> IVGGQECKDGECPWQALLINEENEGFCGGTILSEFYILTAAHCLYQAKRFKVRVGDRN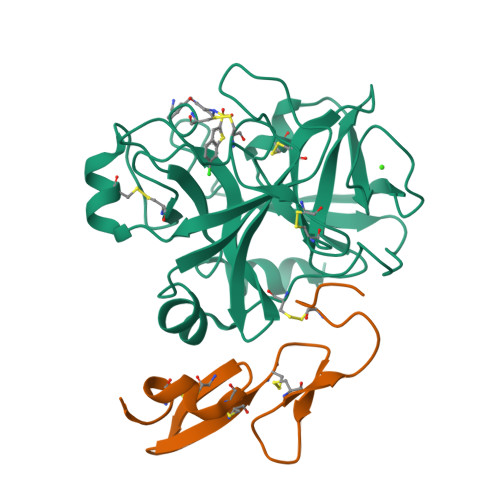TEQEEGGEAVHEVEVVIKHNRFTKETYDFDIAVLRLKTPITFRMNVAPACLPERDWAESTLMTQKTGIVSGFGRTHEKGRQSTRLKMLEVPYVDRNSCKLSSSFIITQNMFCAGYDTKQEDACQGDSGGPHVTRFKDTYFVTGIVSWGEGCARKGKYGIYTKVTAFLKWIDRSMKTRGLPKAKSHAPEVITSSPLK;> EEMKKGHLERECMEETCSYEEAREVFEDSDKTNEFWNKYKDGDQCETSPCQNQGKCKDGLGEYTCTCLEGFEGKNCELFTRKLCSLDNGDCDQFCHEEQNSVVCSCARGYTLADNGKACIPTGPYPCGKQTLERRKRSVAQATSSSGEAPDSITWKPYDAADLDPTENPFDLLDFNQTQPERGDNNLTRIVGGQE(2R)-2-[5-(5-CARBAMIMIDOYL-1H-BENZOIMIDAZOL-2-YL)-6,2'-DIHYDROXY-5'-UREIDOMETHYL-BIPHENYL-3-YL]-SUCCINIC ACID | C26 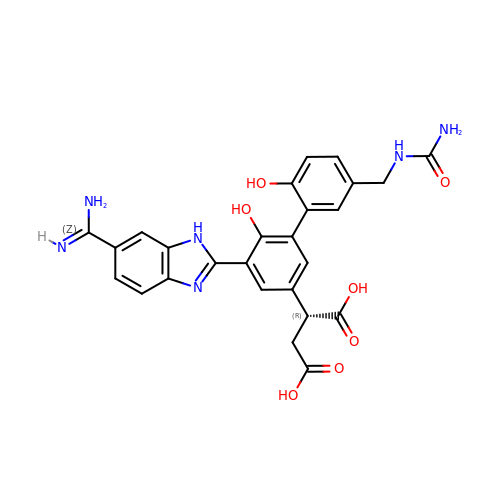H24 N6 O7 | JCBJULMYEXYZRC-CQSZACIVSA-N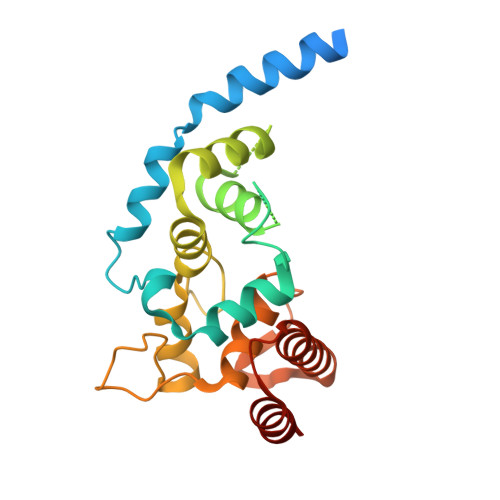> GSHMQPVGKPPKKKKSKRILLKILLTILIIIALFIGIMYFLSTRDNVDELRKIENKSSFVSADNMPEYVKGAFISMEDERFYNHHGFDLKGTTRALFSTISDRDVQGGSTITQQVVKNYFYDNDRSFTRKVKELFVAHRVEKQYNKNEILSFYLNNIYFGDNQYTLEGAANHYFGTTVNKNSTTMSHITVLQSAILASKVNAPSVYNINNMSENFTQRVSTNLEKMKQQNYINETQYQQAMSQLNR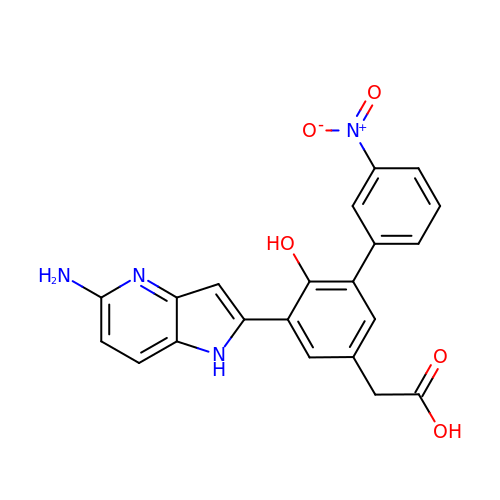{5-(5-AMINO-1H-PYRROLO[3,2-B]PYRIDIN-2-YL)-6-HYDROXY-3'-NITRO-BIPHENYL-3-YL]-ACETIC ACID | C21 H16 N4 O5 | BVBGZXXLVHYBKI-UHFFFAOYSA-N>MRGSHHHHHHTDPHASSVPGRGSIEGRMNNMAGNTPEVVDWFARARRLQKQQLHQLAQQGTLAGQISALVHMLQCERGASNIWLCSGGRLYAAECRAGAALVDEQLTRFYAALEPARDAASSALCWRIACAVWYLPQLAALRKRVRDREIAAEEATGQFSRIIRHLLNIVPQLNDSIDDPQIAGRMVALYSFMQGKELAGQERALGALGFARGQFSDELRQQLVDRIDGQQPCFDSFQALAQPPQTALFAEQCQASLEIEQLRRVACTRQPPADEGETALRWFCAQTQRLEQLRGVEELLIVDLLNAADALLEGEEPEAQLPPADWQEDSIALRLDKQLLPLVRQQAHELQQLSGQLASLKDALEERKLIEKAKSVLMTYQGMQEE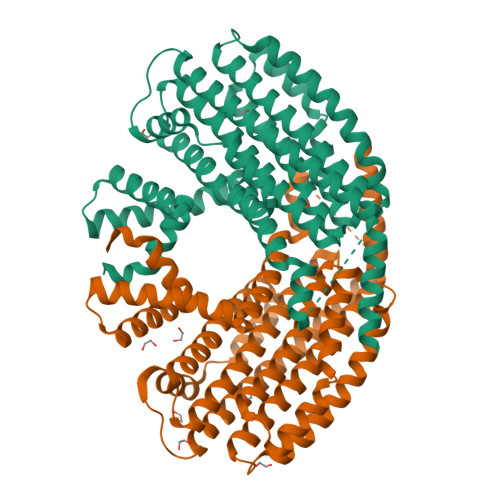QAWQALRKMAMDKNQRMVEIARALLTVKALWRVTPKE[2x]> MLKRLLSKLTGNRQQIEHHLKNQYQVEENGLSFPLSLVDDSQLWALASWLEQLAEEDYLISLTDRWLLSWEALYRLLEDEEHASSLPLIGVPDILPLRASLSSRGALSDSDFRVWIAEWATFPARKPIRFSRTGAILTHDNQQYLLSRENWALLQATEQLSAQQIQTPGETTNQLGWAAIRKCAKLAAAKFDDYLEKTHVIKPTSLSLRLRKATVADTAVIEIEPHFEDQPANWLGSFDKNLQVHDSYRIPGENGELSHVIIPPEVKEVLNSIHSIPGRRVAGSEALSFVRNPYTFLGEDAASVIAPEEHEQALFDARIFFHHFRLIPQLNTENKITEVTLILEPVSPVPQPEITFVFSAPWELDKFIQQLGISVAAQMPAGSWQGYELELSQFTEQQW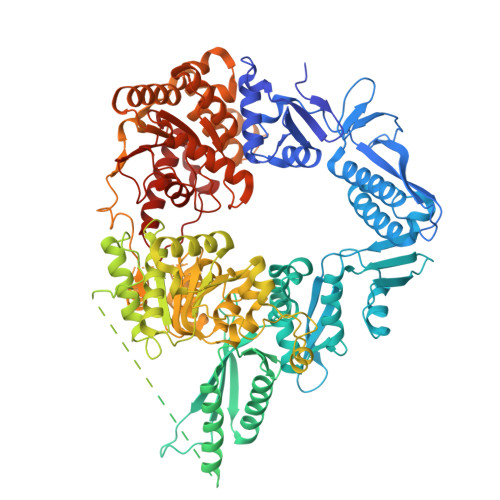HDCQALLTRWQQEIEGKEFSDVLDIAKYGDRVIGIGEFEKISSPWLTKAQSENWLPDGIDFSAFSIETLSGWQPENPLHFDELQEIITQAEAAGETYITTPWNDSQLPLDAAKTFSKNWEKQQITANEYQGNVADKTARAVLKIEQNIEETAYIKQRRNSLLNARHAEPEIPLSLKEHIRLKDHQREGVAWLQQLFLRSPEETAGCLLADDMGLGKTLQILSFLVWFIEKFPQEPPNLIVAPVSLLDNWERELNNFFYTAGIPVLKLYGETIKAVKYPKQAIPAHLQSKGIKNLLKPGWQGEAKIILTTYETLRDQEFSLARQPWSIMVCDEAQKIKNPAALITHAANAVQARFKVACTGTPVENTLVDLWSLFDFAQPGLLGALNEFGKQYVRPIENEDGRDTERLESLRALIEPQTLRRTKEEVARDLPQKIEVESCKQLTLSGVQKQLYLSSVANWQQQQALREGMQQAGTGMLGLLHRLKLICAHPAIVNPEPRFRDNSPKLNWLLKILAEIKHTSKDKVIIFTELRDLQRELQHAIHQNFGFRPVIINGDSSTKSQSQNSRQRLIDDFQAQPGFGVIILSTVAVGFGVNVQKANHVIHFTRCWNPAKEDQATDRAYRIGQTKNVYVYYPTVRDTEITTFEETLDDLLQRRRALARDMLCATPDLNCADFETILKGA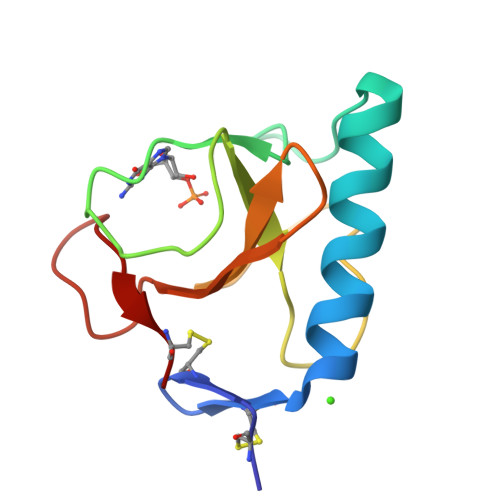> ACDYTCGSNCYSSSDVSTAQAAGYKLHEDGETVGSNSYPHKYNNYEGFDFSVSSPYYAWPILSSGDVYSGGSPGADRVVFNENNQLAGVITHTGASGNNFVECT5-methoxy-2-(4-methoxyphenyl)-3H-indol-3-one 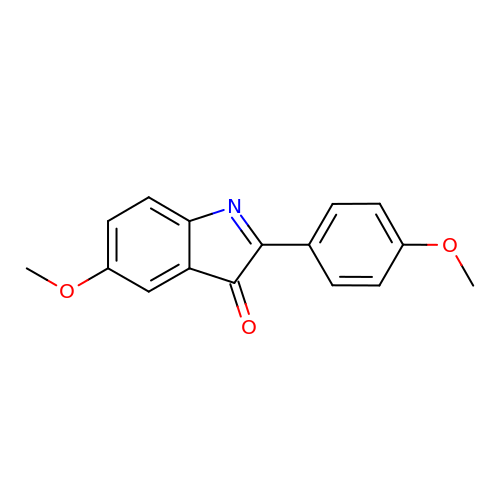| C16 H13 N O3 | VCLRIWYAOAOICS-UHFFFAOYSA-N>[4x]SSPSPLNPGTNVARLAEQAPIHWVSVAQIENSLAGRPPMAVGFDIDDTVLFSSPGFWRGKKTFSPESEDYLKNPVFWEKMNNGWDEFSIPKEVARQLIDMHVRRGDAIFFVTGRSPTK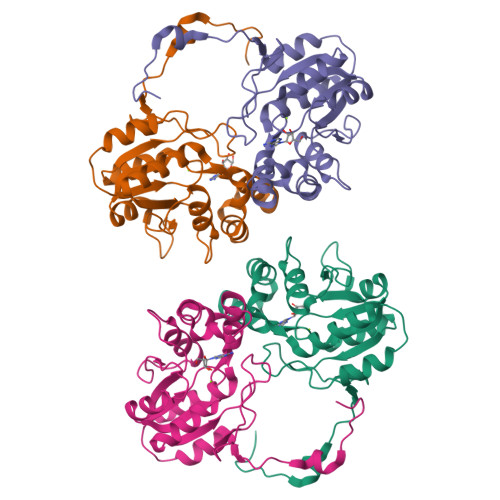TETVSKTLADNFHIPATNMNPVIFAGDKPGQNTKSQWLQDKNIRIFYGDSDNDITAARDVGARGIRILRASNSTYKPLPQAGAFGEEVIVNSEY> SEQNNAVLPKGVTQGEFNKAVQKFRALLGDDNVLVESDQLVPYNKIMMPVENAAHAPSAAVTATTVEQVQGVVKICNEHKIPIWTISTGRNFGYGSAAPVQRGQVILDLKKMNKIIKIDPEMCYALVEPGVTFGQMYDYIQENNLPVMLSFSAPSAIAGPVGNTMDRGVG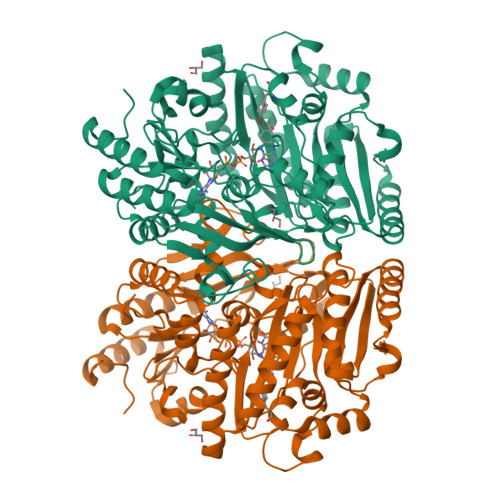YTPYGEHFMMQCGMEVVLANGDVYRTGMGGVPGSNTWQIFKWGYGPTLDGMFTQANYGICTKMGFWLMPKPPVFKPFEVIFEDEADIVEIVDALRPLRMSNTIPNSVVIASTLWEAGSAHLTRAQYTTEPGHTPDSVIKQMQKDTGMGAWNLYAALYGTQEQVDVNWKIVTDVFKKLGKGRIVTQEEAGDTQPFKYRAQLMSGVPNLQEFGLYNWRGGGGSMWFAPVSEARGSECKKQAAMAKRVLHKYGLDYVAEFIVAPRDMHHVIDVLYDRTNPEETKRADACFNELLDEFEKEGYAVYRVNTRFQDRVAQSYGPVKRKLEHAIKRAVDPNNILAPGRSGIDLNNDF>[2x]GHMGSNSLSMIKVRLQNLFDNDEVALLKITCYTDKLIHLTNALAKAVIHTIKLNGIVFVHVITSSDICPNNNIVVKSNFTTMPVLQNGGYIWEMM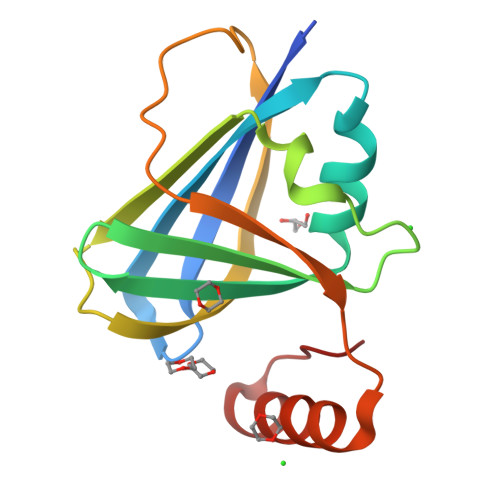ELTHCSQPNGLIDDNCEIKFSKKLSDSTMTNYMNQLSELLGFDLNP>[5x]MEQPINVLNDFHPLNEAGKILIKHPSLAERKDEDGIHWIKSQWDGKWYPEKFSDYLRLHKIVKIPNNSDKPELFQTYKDKNNKRSRYMGLPNLKRANIKTQWTREMVEEWKKCRDDIVYFAETYCAITHIDYGVIKVQLRDYQRDMLKIMSSKRMTVCNLSRQLGKTTVVAIFLAHFVCFNKDKAVGILAHKGSMSAEVLDRTKQAIELLPDFLQPGIVEWNKGSIELDNGSSIGAYASSPDAVRGNSFAMIYIDECAFIPNFHDSWLAIQPVISSGRRSKIIITTTPNGLNHFYDIWTAAVEGKSGFEPYTAIWNSVKERLYNDEDIFDDGWQWSIQTINGSSLAQFRQEHTAAFEGTSGTLISGMKLAVMDFIEVTPDDHGFHQFKKPEPDRKYIATLDCSEGRGQDYHALHIIDVTDDVWEQVGVLHSNTIS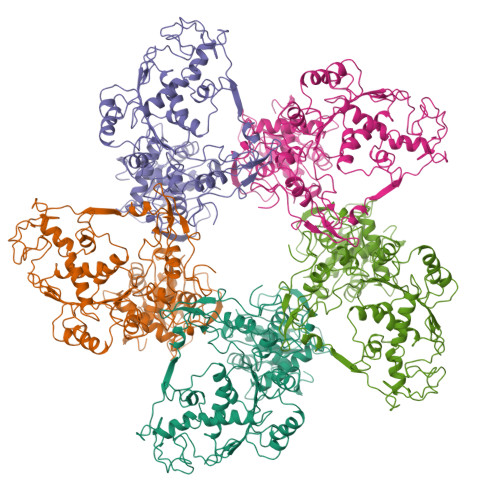HLILPDIVMRYLVEYNECPVYIELNSTGVSVAKSLYMDLEYEGVICDSYTDLGMKQTKRTKAVGCSTLKDLIEKDKLIIHHRATIQEFRTFSEKGVSWAAEEGYHDDLVMSLVIFGWLSTQSKFIDYADKDDMRLASEVFSK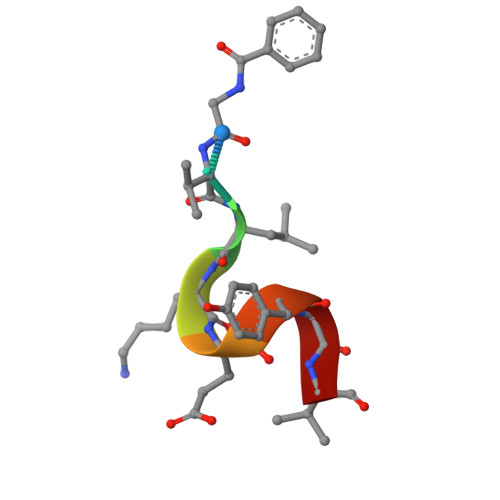> XVLKEYGV>MPVRRGHVAPQNTFLDTIIRKFEGQSRKFIIANARVENCAVIYCNDGFCELCGYSRAEVMQRPCTCDFLHGPRTQRRAAAQIAQALLGAEERKVEIAFYRKDGSCFLCLVDVVPVKNEDGAVIMFILNFEVVMEKDMVGSGADVLPEYKLQAPRIHRWTILHYSPFKAVWDWLILLLVIYTAVFTPYSAAFLLKETEEGPPATECGYACQPLAVVDLIVDIMFIVDILINFRTTYVNANEEVVSHPGRIAVHYFKGWFLIDMVAAIPFDLLIFGSGSEELIGLLKTARLLRLVRVARKLDRYSEYGAAVLFLLMCTFALIAHWLACIWYAIGNMEQPHMDSRIGWLHNLGDQIGKPYNSSGLGGPSIKDKYVTALYFTFSSLTSVGFGNVSPNTNSEKIFSICVMLIGSLMYASIFGNV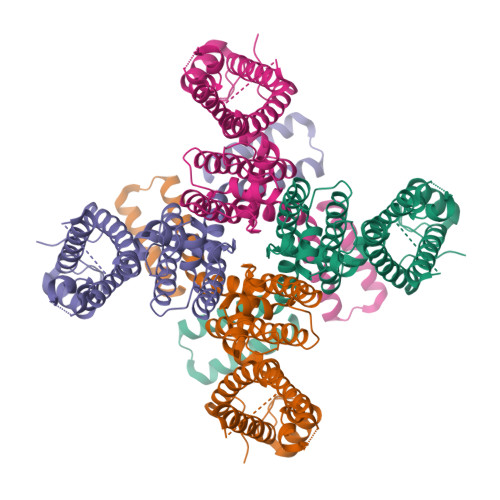SAIIQRLYSGTARYHTQMLRVREFIRFHQIPNPLRQRLEEYFQHAWSYTNGIDMNAVLKGFPECLQADICLHLNRSLLQHCKPFRGATKGCLRALAMKFKTTHAPPGDTLVHAGDLLTALYFISRGSIEILRGDVVVAILGKNDIFGEPLNLYARPGKSNGDVRALTYCDLHKIHRDDLLEVLDMYPEFSDHFWSSLEITFNLRDTNMIPGGRQYQELPRCPAPTPSLLNIPLSSPGRRPRGDVESRLDALQRQLNRLETRLSADMATVLQLLQRQMTLVPPAYSAVTTPGPGPTSTSPLLPVSPLPTLTLDSLSQVSQFMACEELPPGAPELPQEGPTRRLSLPGQLGALTSQPLHRHGSDPGS[4x]> GAMVSPPQVDPQ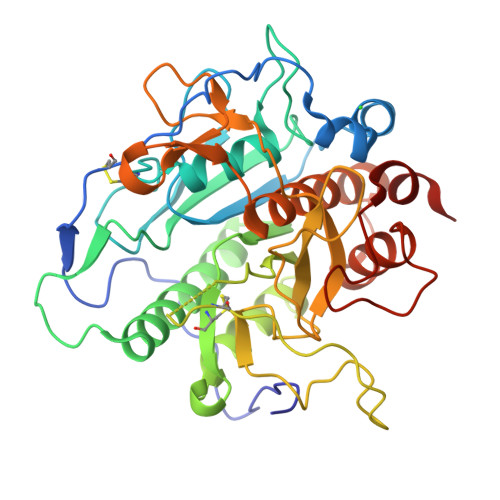IAPPPGTAGPAQPMMQRSECITTSVLPGTDPGAVSPNQLALNLSGAWQHSRGAGQTVAVIDTGVQPGPRLPNVEAGGDYIESTDGLTDCDGHGTSVAGLIAGQPGPDGFSGVAPEARLISIRQNSPRFAPRTPGADSEATRAASDAETLARAVVRAADMGARVINISLVTCLPADRTIDQSVLGAALRYAALEKDAVIVAAAGNNRGGVSTGAACESNPLPSGTPGDPRNWNGVTSVSIPSWWQPYVLSVGAVDSTGQPSSFTMAGPWVGIAAPGENIVSVSNAPDGGLSNALPSERDRLVPLTGTSYAAAYVSGVAALVRSKFPDLTARQVVHRLTTTAQGAARSPSNLIGAGMVDPVAALTWDVADV Four helix bundles are also attractive for synthetic chemists because its interfaces are dominated by side chain and side chain interactions, which can be more tunable than β-strands. This study focuses on TmFtn, a naturally dimeric protein consisting of two antiparallel four helix bundles, as shown in Supplementary Fig. 1. Thermotoga maritima ferritin (TmFtn) naturally occurs as a dimer; twelve of these dimers interact with each other in a head-to-side manner to generate 24-meric hollow protein nanocage in the presence of Ca2+ or PEG. By tuning two contiguous dimeric proteins to interact in a fully or partially side-by-side fashion through protein interface redesign, we can render the self-assembly transformation of such dimeric building blocks from the protein nanocage to filament, nanorod and nanoribbon in response to multiple external stimuli.

The crystal structure analyses revealed that FLAL-L molecules are perfectly aligned with each other in a partially side-by-side manner to form filaments, the top view of which is in good agreement with the filament observed under TEM. As expected, intermolecular associations between two adjacent FLAL-L molecules are mediated entirely through hydrophobic interactions, as the contact region of adjacent FLAL-L molecules is rich in hydrophobic amino acid residues. The engineered Leu114 and Leu137 side chains cooperated with the original V119, L107, V126, and V130 side chains provide the bulk of the hydrophobic core, whereas the engineered Leu112, Ala113, and Phe147 are not involved in such interactions. The crystal structure provides direct evidence to confirm the partially side-by-side manner of FLAL-L molecules. The above formed filaments coalesce in parallel along the y axes through hydrogen bonds, leading to the generation of a protein layer, corresponding to the ribbons observed by TEM. In crystals, the formed protein layers further arrange along the z axes to form 3D protein frameworks through π–π interactions and electrostatic interactions. The significant difference in self-assembly behavior between these two dimeric protein molecules reflects the importance of amino acid residue Arg137 in FLAL, suggesting that Arg137 could act as a switch to control the conversion of nanorods to nanoribbons.

>[3x]MMVISEKVRKALNDQLNREIYSSYLYLSMATYFDAEGFKGFAHWMKKQAQEELTHAMKFYEYIYERGGRVELEAIEKPPSNWNGIKDAFEAALKHEEFVTQSIYNILELASLALDHATVSFLKWFVDEQVEEEDQVLEILDLLEKAFGQMSVIFQLDRYLGQRE(5R)-6-acetyl-2-methoxy-N-{4-[(2-methoxyphenyl)methoxy]phenyl}-5,6,7,8-tetrahydro-1,6-naphthyridine-5-carboxamide 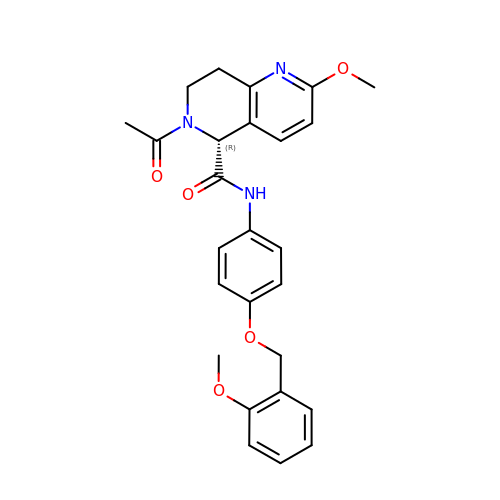| C26 H27 N3 O5 | RNCVXSNHCXEILI-RUZDIDTESA-N>[3x]MRLPRETDEEPEEPGRRGSFVEMVDNLRGKSGQGYYVEMTVGSPPQTLNILVDTGSSNFAVGAAPHPFLHRYYQRQLSSTYRDLRKGVYVPYTQGKWEGELGTDLVSIPHGPNVTVRANIAAITESDKFFINGSNWEGILGLAYAEIARPDDSL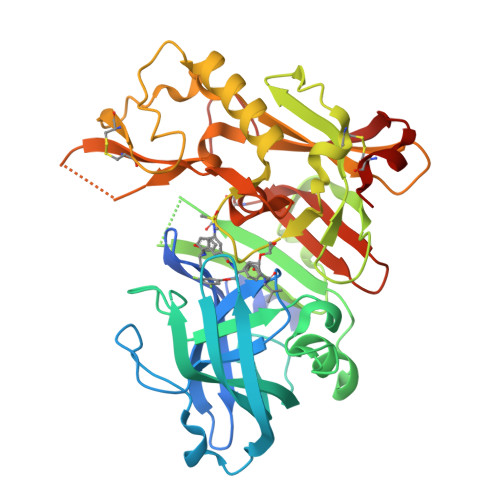EPFFDSLVKQTHVPNLFSLQLCGAGFPLNQSEVLASVGGSMIIGGIDHSLYTGSLWYTPIRREWYYEVIIVRVEINGQDLKMDCKEYNYDKSIVDSGTTNLRLPKKVFEAAVKSIKAASSTEKFPDGFWLGEQLVCWQAGTTPWNIFPVISLYLMGEVTNQSFRITILPQQYLRPVEDVATSQDDCYKFAISQSSTGTVMGAVIMEGFYVVFDRARKRIGFAVSACHVHDEFRTAAVEGPFVTLDMEDCGYN>MKILVIEDDALLLQGLILAMQSEGYVCDGVSTAHEAALSLASNHYSLIVLDLGLPDEDGLHFLSRMRREKMTQPVLILTARDTLEDRISGLDTGADDYLVKPFALEELNARIRALLRRHNNQGDNEISVGNLRLNVTRRLVWLGETALDLTPKEYALLSRLMMKAGSPVHREILYNDIYSGDNEPATNTLEVHIHNLREKIGKSRIRTVRGFGYMLANNDDTEHLEHHHHHH[2x]

The PmrA/PmrB TCS is a major regulator of genes for lipopolysaccharide modification in the outer membrane of bacteria. The response regulator PmrA, which belongs to the OmpR/PhoB family, functions as a transcription factor. Each OmpR/PhoB member contains an N-terminal receiver domain (REC) and a C-terminal DNA-binding domain (DBD), connected by a linker. Here, we determine the crystal structure of BeF3−-activated PmrA in complex with the promoter DNA, which also reveals a REC–DBD interface in the upstream protomer, but the interactions of the interface are notably different from those observed in the KdpE–DNA complex structure.

We reveal the crystal structures of BeF3−-activated PmrA in complex with 25-bp DNA at 3.2 Å resolution and with 26-bp DNA at 3.8 Å resolution. The PmrA–26-bp DNA crystal has only one copy of the protein–DNA complex (complex-3) packed in a different space group, P3121. All the three complex structures contain a BeF3−-activated PmrA dimer (residues 1–219 modelled) binding to a double-stranded DNA (The upstream protomer that recognizes half-1 site is denoted PmrA-1 and the downstream protomer PmrA-2.) with similar conformations. R.m.s.d. values between the three complex structures decreased to 0.6–1.0 Å with the PmrA-2 DBD excluded. Complex-2 and complex-3 feature similar interactions between the two DBDs, with interfaces of 303.7 and 284.1 Å2, respectively. The interface interactions identified in the three complexes are also similar. Similar crystal structures are obtained from two crystals of distinct shapes and space groups, growing with different lengths of DNA in different conditions, which rules out the possibility of a crystal packing effect.2-[[4-(6-bromanyl-2~{H}-indazol-4-yl)-1,2,3-triazol-1-yl]methyl]-6-[(4,4-dimethylpiperidin-1-yl)methyl]imidazo[1,2-a]pyridine | C25 H27 Br N8 | 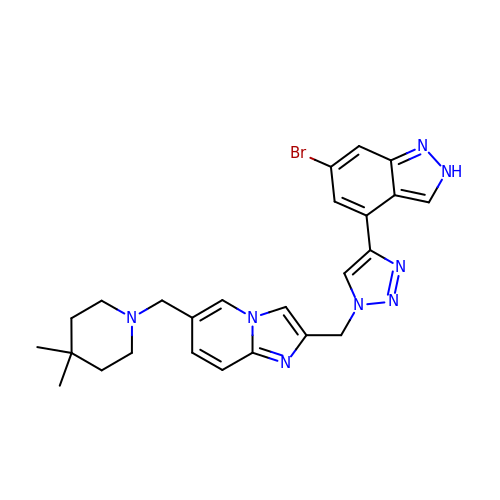RXIOMUYKKTZDFQ-UHFFFAOYSA-N>[3x]ATDAASLVGELQAADAEYQNLAN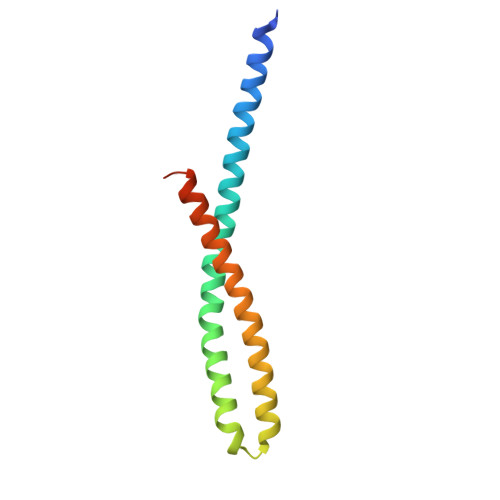QEEARFNEERAQADAARQALAQNEQVYNELSQRAQRLQAEANTRFYKSQYQELASKYEDALKKLEAEMEQQKAVISDFEKIQALRAGNLEHHHHHH> MSLHEKMQTDYLWVKDHSQADSWAKARTHGYNYIAHTVPNKKERYEMIWRSMGKSTDWELEKFRLGKKFPDRGNKRRWFKNLFRLIKNPMGYIFWKTYKARLAKPSLIV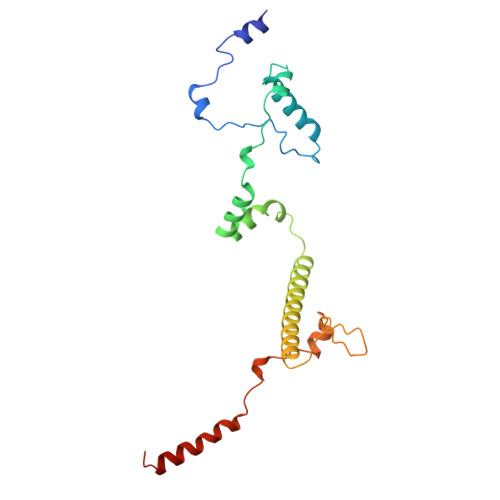TSMFIGFTLGFIKLKAQSIAYSKKQYATLRAGKNIEGSGQVHFGYHDQKWGMPAIPMFQLMYYELPGNSIVVNPCRNQNYRLYFEMRKKLGILPA2-[4-(ethylsulfonyl)phenyl]-N-{5-[2-(2-methylpropyl)benzoyl]-4-phenyl-1,3-thiazol-2-yl}acetamide 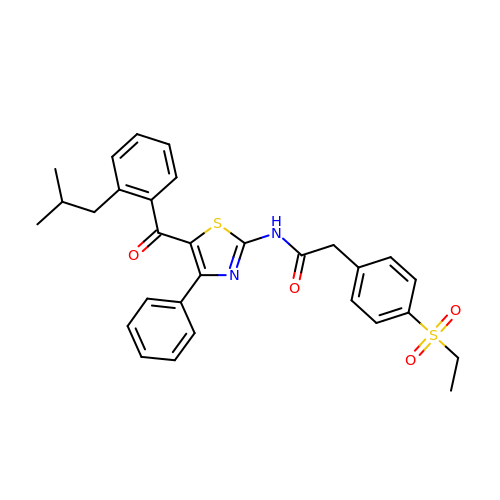| C30 H30 N2 O4 S2 | JCEZUYLHQPJLPN-UHFFFAOYSA-N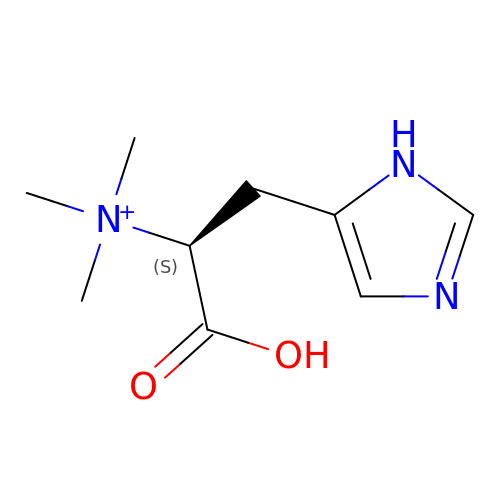N,N,N-trimethyl-histidine | C9 H16 N3 O2 | GPPYTCRVKHULJH-QMMMGPOBSA-O>[4x]HLLQFRKMIKKMTGKEPVVSYAFYGCYCGSGGRGKPKNATDRCCFVHDCCYE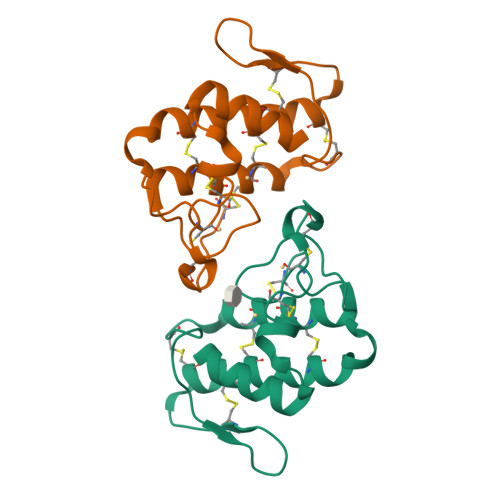KVTGCDPKWDDYTYSWKNGTIVCGGDDPCKKEVCECDKAAAICFRDNLKTYKKRYMAYPDILCSSKSEKC>GSKKRPKPGGWNTGGSRYPGQGSPGGNRYPPQGGTWGQPHGGGWGQPHGGSWGQPHGGSWGQPHGGGWGQGGGTHNQWNKPSKPKTNLKHVAGA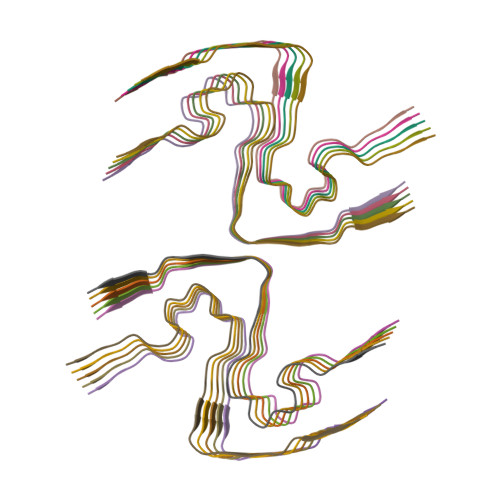AAAGAVVGGLGGYMLGSAMSRPMIHFGND[20x]>[12x]SNAMDSNTMSSFQVDCFLWHIRKRFADNGLGD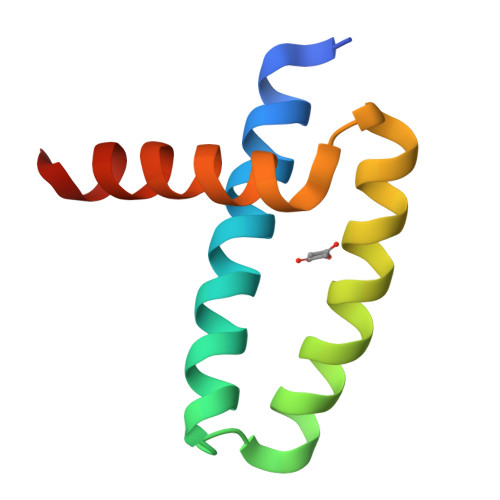APFLDRLRRDQKSLKGRGNTLGLDIETATLVGKQIVEWILKEES> GLPVMNTPGSNQFLTSDDFQSPSAMPQFDVTPELNIPGEVQNLMEIAEVDSVVPVNNVEGKLDTMEIYRIPVQSGNHQSSQVFGFQVQPGLDNVFKHTLLGEILNYYAHWSGSIKLTFVFCGSAMATGKFLLAYAPPGANAPKSRKDAMLGTHIIWDVGLQSSCVLCIPWISQTHYRLVQQDEYTSAGNVTCWYQTGIVVPAGTPTSCSIMCFVSACNDFSVRLLKDT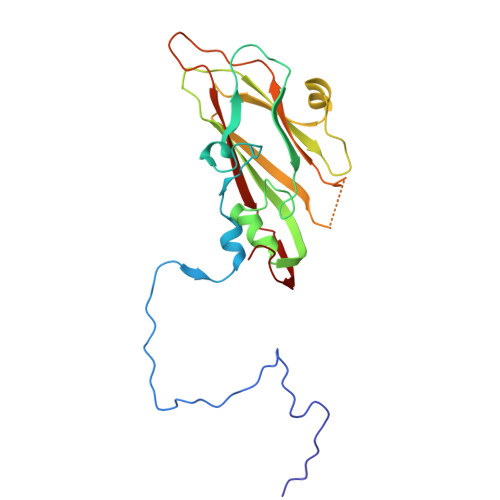PFI>MEEPEEPA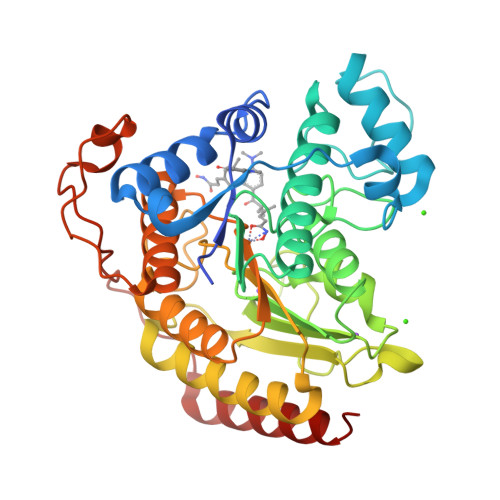DSGQSLVPVYIYSPEYVSMCDSLAKIPKRASMVHSLIEAYALHKQMRIVKPKVASMEEMATFHTDAYLQHLQKVSQEGDDDHPDSIEYGLGYDCPATEGIFDYAAAIGGATITAAQCLIDGMCKVAINWSGGWHHAKKDEASGFCYLNDAVLGILRLRRKFERILYVDLDLHHGDGVEDAFSFTSKVMTVSLHKFSPGFFPGTGDVSDVGLGKGRYYSVNVPIQDGIQDEKYYQICESVLKEVYQAFNPKAVVLQLGADTIAGDPMCSFNMTPVGIGKCLKYILQWQLATLILGGGGYNLANTARCWTYLTGVILGKTLSSEIPDHEFFTAYGPDYVLEITPSCRPDRNEPHRIQQILNYIKGNLKHVV[2x]>MAGRWLDPLWAPGFLCVALILETASGAGDLSTKAHGHIQFSARGVNQTAMADCRAVCSLNTSDRCDFVKRNPDCHSEGGYLDYLKGIFCY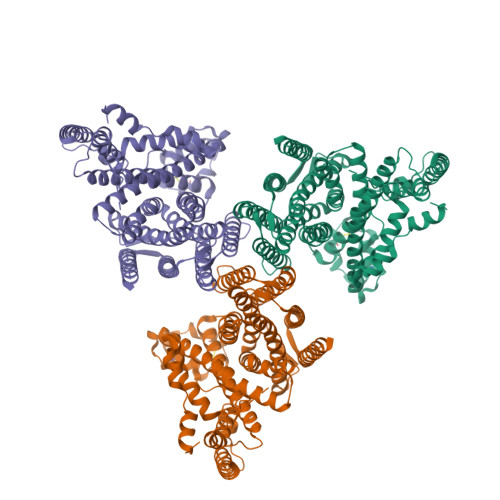FPPNLLPLAITLYVFWLLYLFLILGVTAAKFFCPNLSAISTSLKLSHNVAGVTFLAFGNGAPDIFSALVAFSDPRTAGLAIGALFGAGVLVTTVVAGGITILRPFMAASRPFLRDITFYMVAVFLTFTALYLGRITLVWALGYLGLYVFYVVTVIICTWVYQRQRSRSLVHSISETPELLTDSEEDQMSSNTNSYDYGEEYRPLLLGEETTGQILLQALNPLDYRKWRTQSISCKLLKVAKLPVEFLLLLTVPVVDPDKDDRNWKRPLNCLQLVISPLVLVLTLQSGVYGIYEIGGLLPVWAVVVIVGTALASVTFFATSNSEPPRLHWLFAFLGFLTSALWINAAATEVVNILRSLGVVFRLSNTVLGLTLLAWGNSIGDAFSDFTLARQGYPRMAFSACFGGIIFNILVGVGLGCLLQIVRSHASEVKLEPDGLLVWVLASALGLSLVFSLVSVPLQCFQLSKAYGLCLLLFYICFIVVVLLTEFGVIHLKAD[3x]>[2x]HHHHSGDDDDSQPRADKPSQLKKPRWKRVPTREENVIQC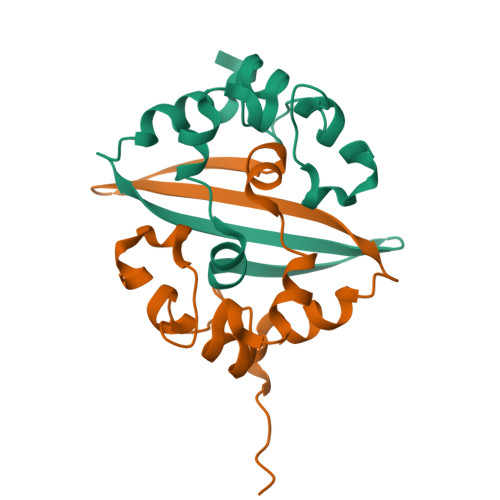FGPRDFNHNMGDSDLVQNGVDAKGFPQLAELIPNQAALFFDSEVSTDEVGDNVQITYTYKMLVAKDNKNLPKFIEQISAFTKPSSIKEMQS> CGCAI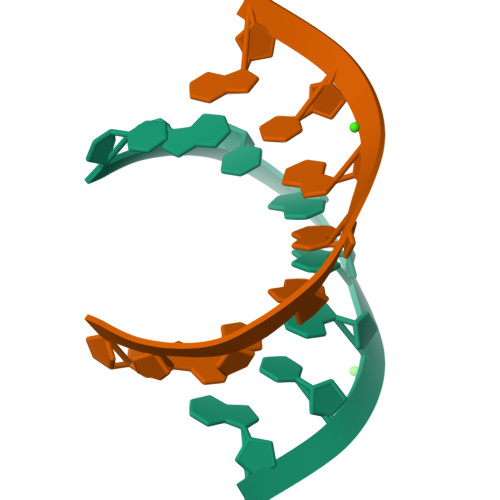GCG>[2x]MNILLCCSAGMSTS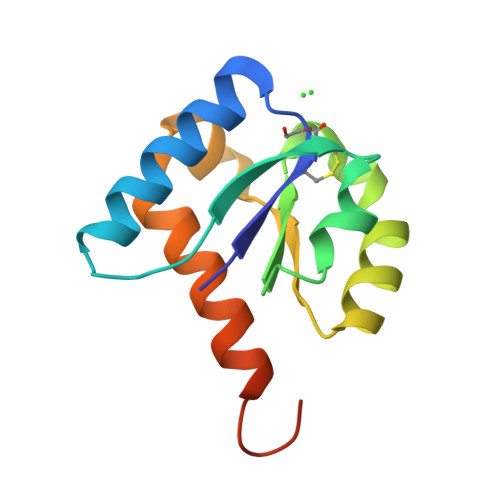LLVTKMEAAAKARGLEGKIWAVSGDAVKTNIDQADVLLLGPQVRYMLSSMKTLADERNVGIDVINPMHYGMMNGEAVLDHALTLKKGENLYFQSAGHHHHHH> MERPWGAADGLSRWPHGLGLLLLLQLLPPSTLSQDRLDAPPPPAAPLPRWSGPIGVSWGLRAAAAGGAFPRGGRWRRSAPGEDEECGRVRDFVAKLANNTHQHVFDDLRGSVSLSWVGDSTGVILVLTTFHVPLVIMTFGQSKLYRSEDYGKNFKDITDLINNTFIRTEFGMAIGPENSGKVVLTAEVSGGSRGGRIFRSSDFAKNFVQTDLPFHPLTQMMYSPQNSDYLLALSTENGLWVSKNFGGKWEEIHKAVCLAKWGSDNTIFFTTYANGSCKADLGALELWRTSDLGKSFKTIGVKIYSFGLGGRFLFASVMADKDTTRRIHVSTDQGDTWSMAQLPSVGQEQFYSILAANDDMVFMHVDEPGDTGFGTIFTSDDRGIVYSKSLDRHLYTTTGGETDFTNVTSLRGVYITSVLSEDNSIQTMITFDQGGRWTHLRKPENSECDATAKNKNECSLHIHASYSISQKLNVPMAPLSEPNAVGIVIAHGSVGDAISVMVPDVYISDDGGYSWTKMLEGPHYYTILDSGGIIVAIEHSSRPINVIKFSTDEGQCWQTYTFTRDPIYFTGLASEPGARSMNISIWGFTESFLTSQWVSYTIDFKDILERNCEEKDYTIWLAHSTDPEDYEDGCILGYKEQFLRLRKSSMCQNGRDYVVTKQPSICLCSLEDFLCDFGYYRPENDSKCVEQPELKGHDLEFCLYGREEHLTTNGYRKIPGDKCQG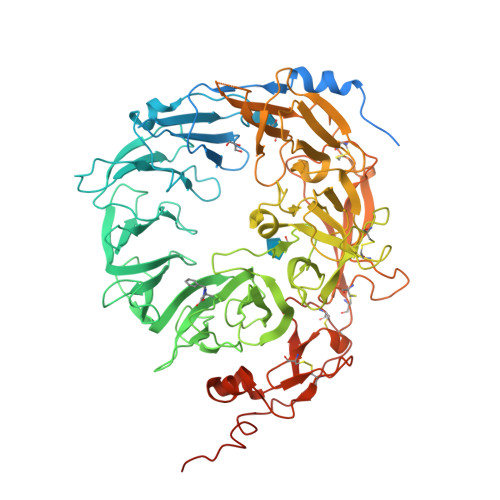GVNPVREVKDLKKKCTSNFLSPEKQNSKSNSHHHHHH>METDLNSQDRKDLDKFIKFFALKTVQVIVQARLGEKICTRSSSSPTGSDWFNLAIKDIPEVTHEAKKALAGQLPAVGRSMCVEISLKTSEGDSMELEIWCLEMNEKCDKEIKVSYTVYNRLSLLLKSLLAITRVTPAYRLSRKQGHEYVILYRIYFGEVQLSGLGEGFQTVRVGTVGTPVGTITLSCAYR[2x];>MNCRSEVLEVSVEGRQVEEAMLAVLHTVLLHRSTGKFHYAAAGTYSIGTVGTQDVDCDFIDFTYVRVSSEELDRALRKVVGEFKDALRNSGGDGLGQMSLEFYQKKKSRWPFSDECIPWEVWTVKVHVVALATEQERQICREKVGEKLCEKIINIVEVMNRHEYLPKMPTQSEVDNVFDTGLRDVQPYLYKISFQITDALGTSVTTTMRRLIKDT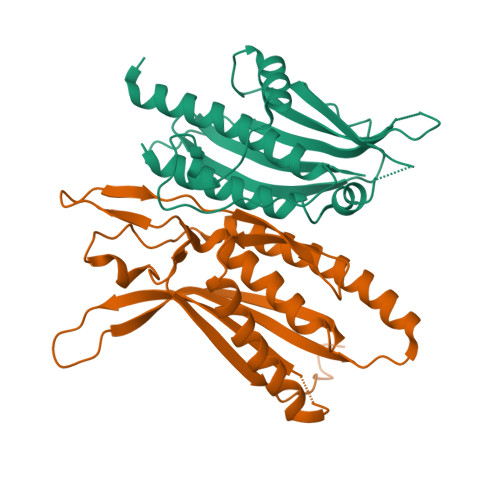LAL[2x]>MNSQLTLRALERGDLRFIHNLNNNRNIMSYWFEEPYESFDELEELYNKHIHDNAERRFVVEDAQKNLIGLVELIEINYIHRSAEFQIIIAPEHQGKGFARTLINRALDYSFTILNL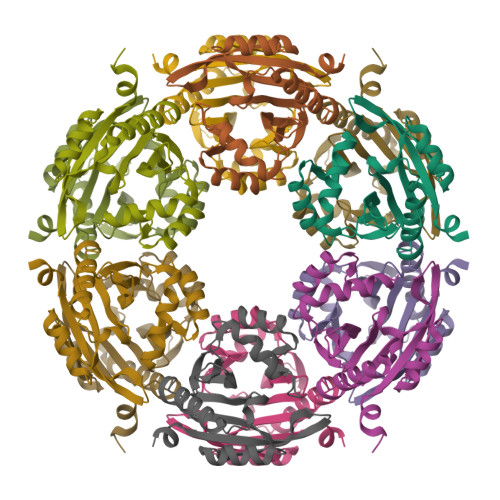HKIYLHVAVENPKAVHLYEECGFVEEGHLVEEFFILGRYQDVKRMYILQSKYLNRSE[3x]2-amino-7-(1,1-dioxo-1lambda~6~-thian-4-yl)-5-oxo-5H-[1]benzopyrano[2,3-b]pyridine-3-carboxylic acid 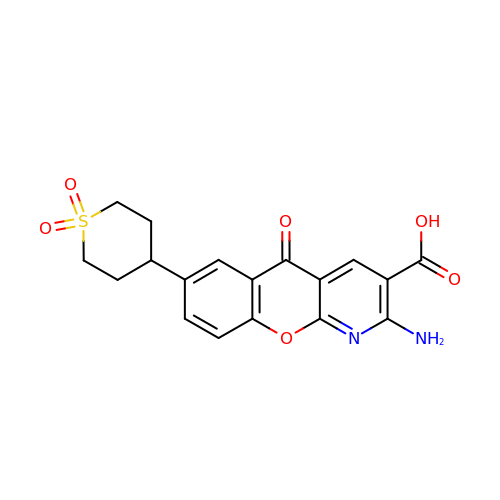| C18 H16 N2 O6 S | YLXHHSZCWBYDQH-UHFFFAOYSA-N> GPVEDAITAAIGRVADTVGTGPTNSEAIPALTAAETGHTSQVVPGDTMQTRHVKNYHSRSESTIENFLCRSACVYFTEYENSGAKRYAEWVITPRQAAQLRRKLEFFTYVRFDLELTFVITSTQQPSTTQNQDAQILTHQIMYVPPGGPVPDKVDSYVWQTSTNPSVFWTEGNAPPRMSIPFLSIGNAYSNFYDGWSEFSRNGVYGINTLNNMGTLYARHVNAGSTGPIKSTIRIYFKPKHVKAWIPRPPRLCQYEK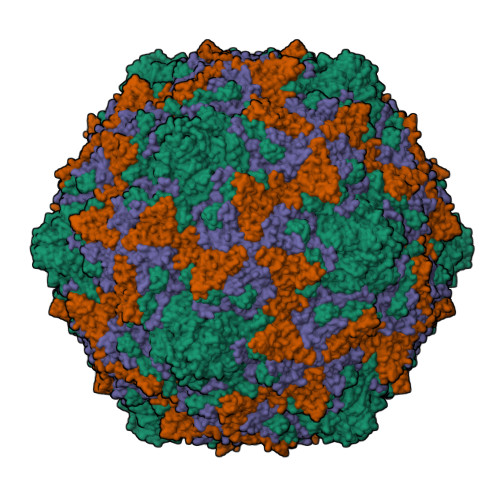AKNVNFQPSGVTTTRQSITTMTNT;> SPTVEECGYSDRVRSITLGNSTITTQECANVVVGYGVWPDYLKDSEATAEDQPTQPDVATCRFYTLDSVQWQKTSPGWWWKLPDALSNLGLFGQNMQYHYLGRTGYTVHVQCNASKFHQGCLLVVCVPEAEMGCATLDNTPSSVELLGGDSAKEFADKPVASGSNKLVQRVVYNAGMGVGVGNLTIFPHQWINLRTNNSATIVMPYTNSVPMDNMFRHNNVTLMVIPFVPLDYCPGSTTYVPITVTIAPMCAEYNGLRLAGHQ;> GLPTMNTPGSCQFLTSDDFQSPSAMPQYDVTPEMRIPGEVKNLMEIAEVDSVVPVQNVGEKVNSMEAYQIPVRSNEGSGTQVFGFPLQPGYSSVFSRTLLGEILNYYTHWSGSIKLTFMFCGSAMATGKFLLAYSPPGAGAPTKRVDAMLGTHVVWDVGLQSSCVLCIPWISQTHYRYVASDEYTAGGFITCWYQTNIVVPADAQSSCYIMCFVSACNDFSVRLLKDTPFITQQNFFQ;> GAQVSTQKTGAHETGLNASGNSIIHYTNINYYKDAASNSANRQDFTQDPGKFTEPVKDIMIKSLPALN4-oxidanyl-~{N}-[(4-phenoxyphenyl)methyl]-2-pyrazol-1-yl-pyrimidine-5-carboxamide | C21 H17 N5 O3 | 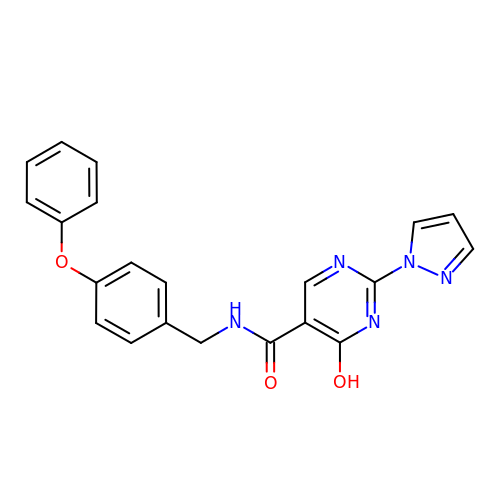WBANHLSPTRNPCR-UHFFFAOYSA-N>GSFTSSNTTTDTSTNSSKKGNVTVTFIPKLTGNAFFESANKGAQKYSEQWGFKVDYEGDANASAASQVSVINKAVQQGTNAICLSSVDAAGVKDALKAAADAGVTVTTWDSDVDPSVRKVMVSQGTPEQLGQMLVQMGYDSLKERG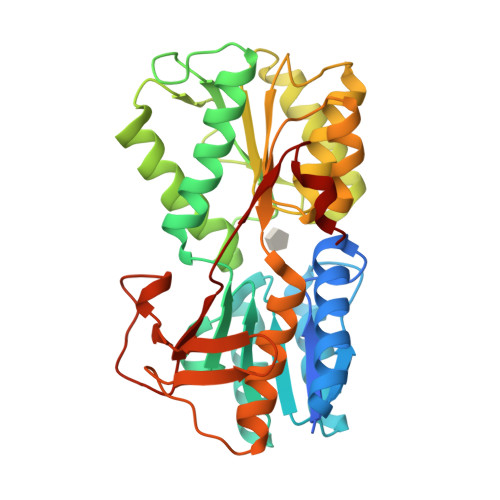KDPEKDAIKYCWHYSNATVTDQNSWQVEGEKYIKSKYPNWQNVAPDNYYSNQDAEQAISVGESILSAHSDIDLIICNDSTALPGQAQAAQNKGLTAKNVTITGFASPNSMKQYCNDGILTRWGLWDCGIQGAMGCYMAYYIASGNSVKVGDKIEIPTVGTVEVMPNSVLDPKADDSDTSSGVVLLPERTIFTKDNMNNYDF[2x]2-[2-[[3-[2,6-bis(chloranyl)phenyl]-5-cyclopropyl-1,2-oxazol-4-yl]methoxy]-6-azaspiro[3.4]octan-6-yl]-1,3-benzothiazole-6-carboxylic 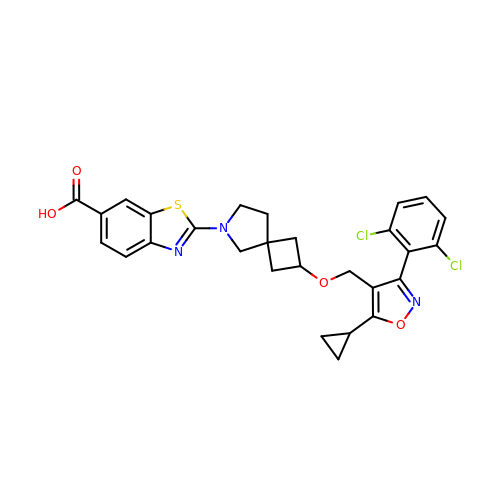acid | C28 H25 Cl2 N3 O4 S | NNWXFKHVPXSNGU-OOTKOPMESA-N>MGASKLRAVLEKLKLSRDDISTAAGMVKGVVDHLLLRLKCDSAFRGVGLLNTGSYYEHVKISAPNEFDVMFKLEVPRIQLEEYSNTRAYYFVKFKRNPKENPLSQFLEGEILSASKMLSKFRKIIKEEINDIKDTDVIMKRKRGGSPAVTLLISEKISVDITLALESKSSWPASTQEGLRIQNWLSAKVRKQLRLKPFYLVPKHAKEGNGFQEETWRLSFSHIEKEILNNHGKSKTCCENKEEKCCRKDCLKLMKYLLEQLKERFKDKKHLDKFSSYHVKTAFFHVCTQNPQDSQWDRKDLGLCFDNCVTYFLQCLRTEKLENYFIPEFNLFSSNLIDKRSKEFLTKQIEYERNNEFPVFD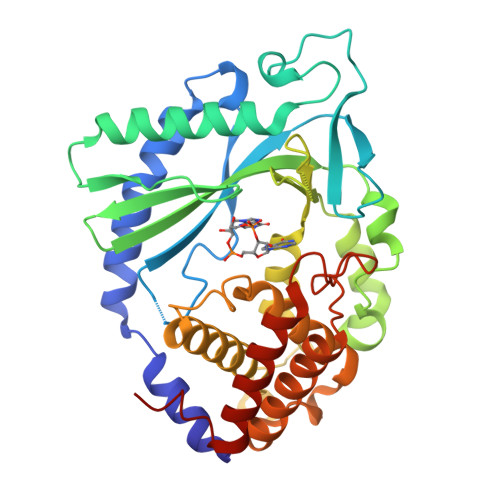EF[2x]> QDNSRYTHFLTQHYDAKPQGRDDRYCESIMRRRGLTSPCKDINTFIHGNKRSI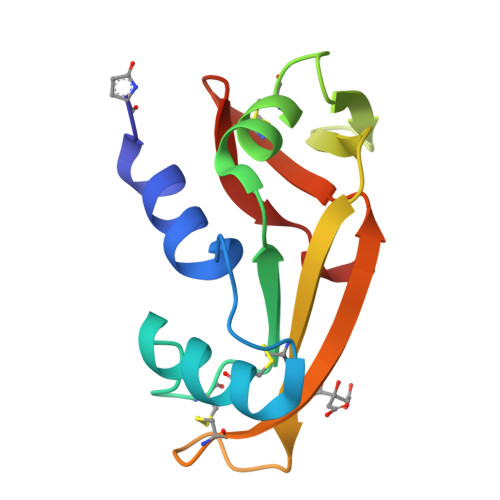KAICENKNGNPHRENLRISKSSFQVTTCKLHGGSPWPPCQYRATAGFRNVVVACENGLPVHLDQSIF Voltage-sensing phosphatases (VSPs) dephosphorylate phosphoinositide (PIP) signaling lipids in response to membrane depolarization. VSPs possess an S4-containing voltage sensor domain (VSD), resembling that of voltage-gated cation channels, and a lipid phosphatase domain (PD). Membrane depolarization drives a rearrangement of S4 that turns on catalytic activity in the PD to dephosphorylate PIPs in the inner leaflet of the membrane. To identify additional coupling determinants, we performed cryogenic electron microscopy (cryo-EM) on the Danio rerio VSP (Dr-VSP) and obtained two structures: a low-resolution monomer structure in a nanodisc and a high-resolution PD dimer structure.

Compared to Ci-VSP, Danio rerio VSP (Dr-VSP) with the active site cysteine mutated to serine (C302S) showed better protein expression and stability. We therefore incorporated Dr-VSP (C302S) into nanodiscs for the study with cryo-EM. One class of particles yielded a structure of the cytoplasmic domain in a dimeric form at a resolution of 3.0 Å. This structure resembled prior X-ray crystal structures of the isolated Ci-VSP cytoplasmic domain15, with the E350 gate (E411 in Ci-VSP) occluding access to the active site (Supplementary Movie-3). The dimeric interface in Dr-VSP buries 744.5 Å2 of surface area and involves 21 residues from each monomer, among which 4 hydrogen bonds (E251/G253, G253/E251, Y261/E461, and E461/Y261) and 5 hydrophobic interactions were observed. A similar, albeit smaller, interface is observed in Ci-VSP crystal structures. While diffuse density was observed in the expected position of the nanodisc and TM region (Supplementary Movie-4), these features were not well resolved in the final map, suggesting flexible attachment in the resting/inactive state. Cryo-EM on Dr-VSP yielded both a high-resolution dimer of the cytoplasmic domain and a low-resolution monomer structure in a nanodisc, which provide structural evidence that a full-length VSP can exist in both monomer and dimer forms. The high-resolution dimer structure reveals residues and interactions that are involved in the dimer formation of the cytoplasmic domain.

>[2x]MTSVHFNPGLDSKEVNGNSVKEEAEVQIGDGKEETKDPDTMYHQVRKKITPFVMSFGFRVFGLVLIILDIIMVIVDLSLSEKSRDVGGALETVSLVISFFFLIDVLLRVYVEGFKVYFSSKLNIVDACIVVITLVVTMIYAFSDFSGASLIPRVVTFLRSLRILILVRIFRLASQKRELEKVTRRMVSENKRRYQKDGFDLDLTYVTERVIAMSFPSSGKQALYRNPIREVVRFLDTKHMDHYKVFNLCSEKGYDPKFFHYRVERVMIDDHNVPSLDDMLRYTACVRDWMAADSRNVIAIHSKGGKGRTGTMVCTWLIDSDQFESAQESLDYFGERRTDKSMSSKFQGVETPSQSRYVGYYEIMKNQYNRQLPPRKSLKIKSIRIHSIAGVGKGNGSDLKLKIIVKHELVFQCVCAKQHNCTVFPDTGSNAVVISLQDGPIVTGDVKVMFESSAGLPKGYEDCPFYFWFNTSFVENYRLFLSREELDNPHKPKTWDIYKEDFGVTLSFTEPSNSLEVLFQ> MASMGRESINPWILTGFADAEGSFSLYIRNTNDRPSRYETRLTFAIGLHYKDKSILENIQSTWKVGIITNAGNNVVQLRVSRFEDLKVIIDHF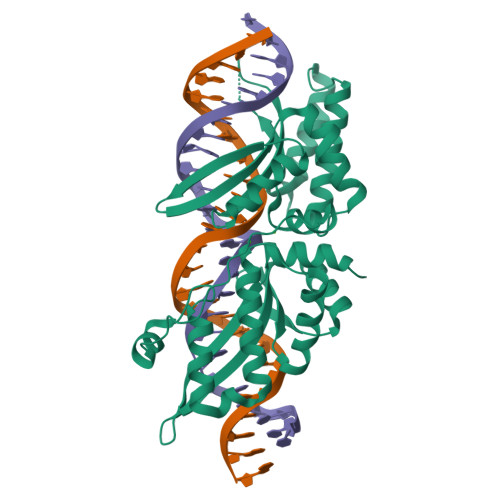EKYPLITQKLGDYKLFKQAFSVMENKEHLKENGIKELVRIKAKMNWGLNDELKKAFPENISKERPLINKNIPNLKWLAGFTSGEGYFGVILAKSRNAATVQVRLRFEIGQHIRDKNLMNSLITYLGCGHIYEKNKSGRSWLVYTVTKFSDISDKIIPVFQKNTLIGVKLEDFEDWCKVAKLIEEKKHLTESGLDEIKKIKLNMNKGRVF(2S,3S,4R,5R,6R)-5-AMINO-2-(AMINOMETHYL)-6-((2R,3R,4R,5S)-5-((1R,2R,3S,5R,6S)-3,5-DIAMINO-2-((2S,3R,4R,5S,6R)-3-AMINO-4,5-DIHYDROXY-6-(HYDROXYMETHYL)-TETRAHYDRO-2H-PYRAN-2-YLOXY)-6-HYDROXYCYCLOHEXYLOXY)-2-(HYDROXYMETHYL)-4-(2-((R)-PIPERIDIN-3-YLMETHYLAMINO)ETHOXY)-TETRAHYDROFURAN-3-YLOXY)-TETRAHYDRO-2H-PYRAN-3,4-DIOL 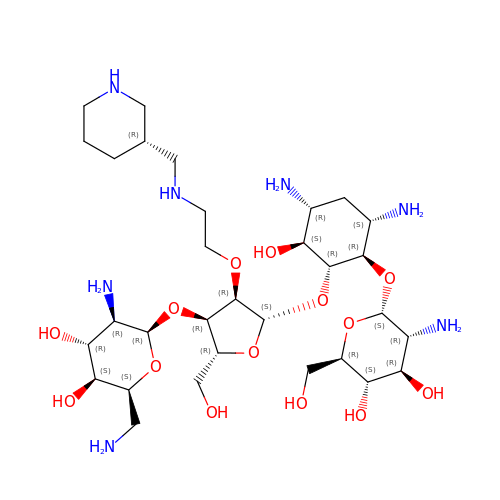| C31 H61 N7 O14 | AHJDGUQMOYBKDU-NSCPTEJBSA-N1-(1-adamantyl)-3-(1-methylsulfonylpiperidin-4-yl)urea | C17 H29 N3 O3 S | 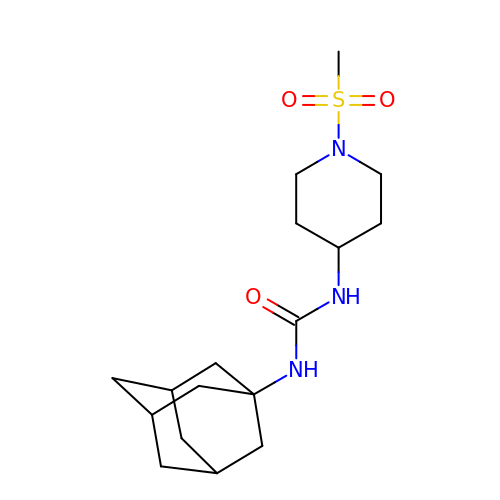DBPGHZGPUBWOQS-ZZNDEYBLSA-N>MTFEEKLSKIYNEIANEISSMIPVEWEKVYTMAYIDDGGGEVFFNYTKPGSDDLNYYTNIPKEYNISVQVFDDLWMDLYDLFEELRDLFKEEDLEPWTSCEFDFTREGELKVSFDYIDWINSEFGQIGR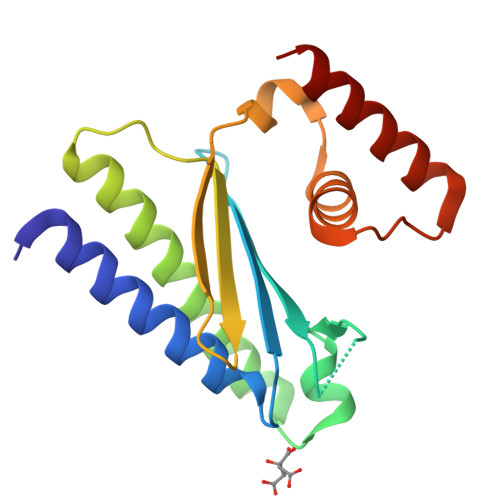QNYYKYRKFGILPETEYEINKVKEIEQYIKELE[2x]[(1~{R})-1-[[(2~{S})-2-[[2,5-bis(chloranyl)phenyl]carbonylamino]-3-(1~{H}-indol-3-yl)propanoyl]amino]-3-methyl-butyl]boronic acid | C23 H26 B Cl2 N3 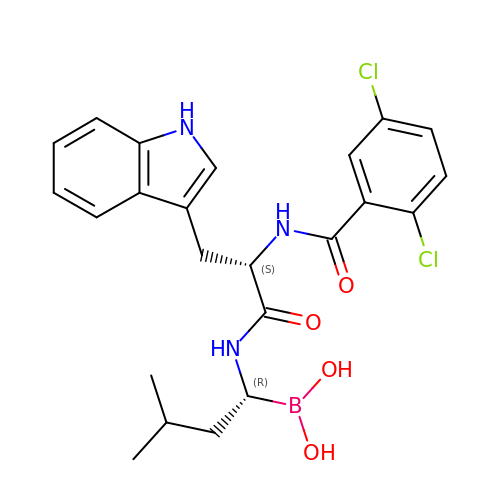O4 | OIYFPOOZLADOLC-SFTDATJTSA-N> MTESYDVVVVGGGPVGLATAWQVAERGHRVLVLERHTFFNENGGTSGAERHWRLQYTQEDLFRLTLETLPLWRALESRCERRLIHEIGSLWFGDTDVVTNEGQISGTAAMMDKLSVRYEWLKATDIERRFGFRGLPRDYEGFLQPDGGTIDVRGTLAALFTLAQAAGATLRAGETVTELVPDADGVSVTTDRGTYRAGKVVLACGPYTNDLLEPLGARLAYSVYEMAIAAYRQATPVTEAPFWFAFQQPTPQDTNLFYGFGHNPWAPGEFVRCGPDFEVDPLDHPSAATGV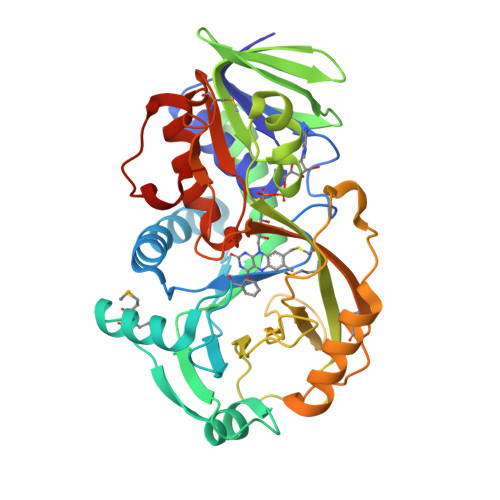ADRRQMDRLSGWLRDHLPTVDPDPVRTSTCLAVLPTDPERQFFLGTARDLMTHGEKLVVYGAGWAFKFVPLFGRICADLAVEDSTAYDISRLAPQALEHHHHHH> FYIETKLDGERMQMHKDGDVYKYFSRNGYNYTDQFGASPTEGSLTPFIHNAFKADIQICILDGEM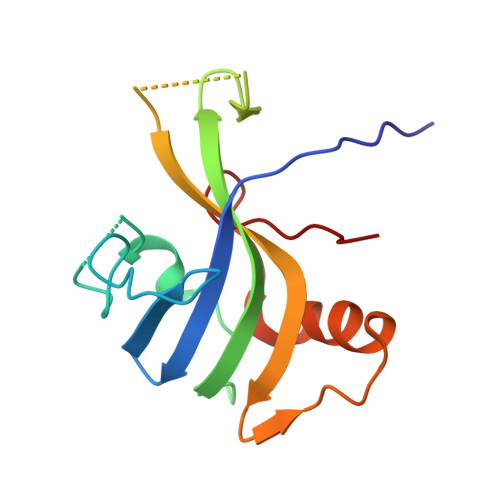MAYNPNTQTFMQKGTKFDIKRMVEDSDLQTCYCVFDVLMVNNKKLGHETLRKRYEILSSIFTPIPGRIEIVQKT>[4x]MAKKTSSKGKLPPGPLPLPGLGNLLHVDFQNTPYCFDQLRRRFGDVFSLQLAWTPVVVLNGLAAVREALVTHGEDTADRPPVPIT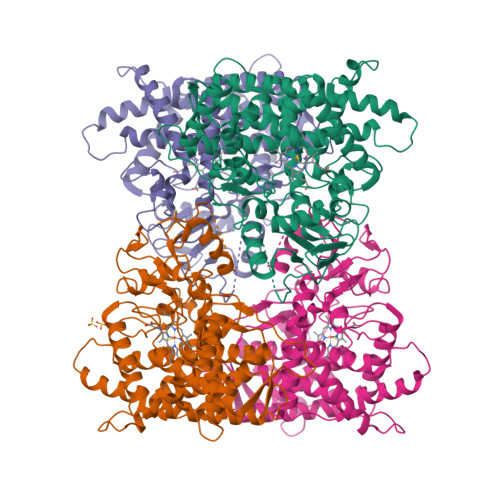QILGFGPRSQGVFLARYGPAWREQRRFSVSTLRNLGLGKKSLEQWVTEEAACLCAAFANHSGRPFRPNGLLDKAVSNVIASLTCGRRFEYDDPRFLRLLDLAQEGLKEESGFLREVLNAVPVDRHIPALAGKVLRFQKAFLTQLDELLTEHRMTWDPAQPPRDLTEAFLAEMEKAKGNPESSFNDENLRIVVADLFSAGMVTTSTTLAWGLLLMILHPDVQRRVQQEIDDVIGQVRRPEMGDQAHMPYTTAVIHEVQRFGDIVPLGMTHMTSRDIEVQGFRIPKGTTLITNLSSVLKDEAVWEKPFRFHPEHFLDAQGHFVKPEAFLPFSAGRRACLGEPLARMELFLFFTSLLQHFSFSVPTGQPRPSHHGVFAFLVSPSPYELCAVPRHHHH6-amino-2-[(thiophen-2-ylmethyl)amino]-1,7-dihydro-8H-imidazo[4,5-g]quinazolin-8-one | C14 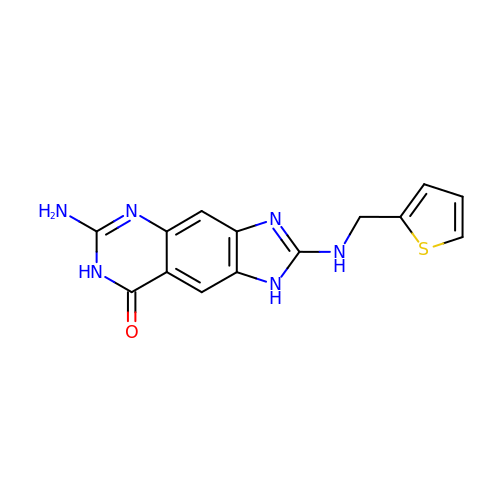H12 N6 O S | IQKMJWDYMFWZRF-UHFFFAOYSA-N>MGIPADNLQSRAKASFDTRVAAAELALNRGVVPSFANGEELLYRNPDPDNTDPSFIASFTKGLPHDDNGAIIDPDDFLAFVRAINSGDEKEIADLTLGPARDPETGLPIWRSDLANSLELEVRGWENSSAGLTFDLEGPDAQSIAMPPAPVLTSPELVAEIAELYLMALGREIEFSEFDSPKNAEYIQFAIDQLNGLEWFNTPAKLGDPPAEIRRRRGEVTVGNLFRGILPGSEVGPYLSQYIIVGSKQIGSATVGNKTLVSPNAADEFDGEIAYGSITISQRVRIATPGRDFMTDLKVFLDVQDAADFRGFESYEPGARLIRTIRDLATWVHFDALYEAYLNACLILLANGVPFDPNLPFQQEDKLDNQDVFVNFGSAHVLSLVTEVATRALKAVRYQKFNIHRRLRPEATGGLISVNKIAAQKGESIF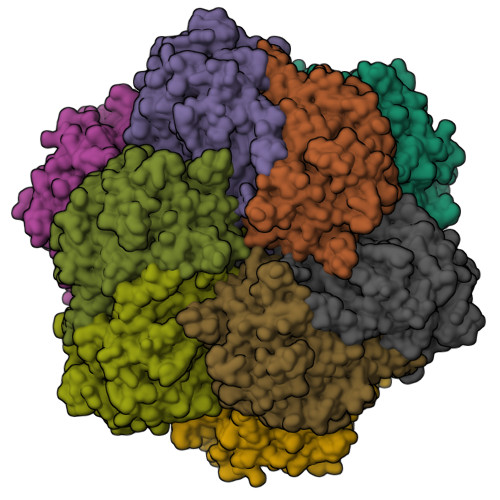PEVDLAVEELGDILEKAEISNRKQNIADGDPDPDPSFLLPMAFAEGSPFHPSYGSGHAVVAGACVTILKAFFDSGIEIDQVFEVDKDEDKLVKSSFKGTLTVAGELNKLADNIAIGRNMAGVHYFSDQFESLLLGEQVAIGILEEQSLTYGENFFFNLPKFDGTTIQI[4x]>[2x]GSHMDSKHQCVKLNDGHFMPVLGFGTYAPPEVPRSKALEVTKLAIEAGFRHIDSAHLYNNEEQVGLAIRSKIADGSVKREDIFYTSKLWSTFHRPELVRPALENSLKKAQLDYVDLYLIHSPMSLKPGEELSPTDENGKVIFDIVDLCTTWEAMEKCKDAGLAKSIGVSNFNRRQLEMILNKPGLKYKPVCNQVECHPYFNRSKLLDFCKSKDIVLVAYSALGSQRDKRWVDPNSPVLLEDPVLCALAKKHKRTPALIALRYQLQRGVVVLAKSYNEQRIRQNVQVFEFQLTAEDMKAIDGLDRNLHYFNSDSFASHPNYPYSDEY

Human aldo–keto reductase 1C3 (AKR1C3; also known as type 5 17β-hydroxysteroid dehydrogenase, prostaglandin F synthase and 3-α-hydroxysteroid dehydrogenase type 2) is a member of the AKR superfamily of NAD(P)H-dependent oxidoreductases that catalyzes the reduction of a diverse range of carbonyl containing substrates, including exogenous compounds and therapeutic drugs. AKR1C3 functions primarily as a 17-ketosteroid reductase that catalyzes NADPH-dependent reduction of weaker steroid hormones to more potent androgens and estrogens: including the reduction of androstenedione to testosterone, 5α-androstanedione to 5α-dihydrotestosterone (DHT) and estrone to 17β-estradiol. AKR1C3 is overexpressed in prostate cancer and most breast cancer types, which makes it an excellent target for the treatment of hormone-dependent cancers. Gatekeeper residues (W227 and L54) in the steroid channel determine substrate orientation, while the oxyanion site, consisting of the nicotinamide ring from the NAD(P)H cofactor and catalytic residues H117 and Y55, anchors ketone, carboxyl or alcohol containing substrates in proximity to the cofactor for enzymatic reactions.

As can be seen, under the assay conditions used, compound 2 inhibits AKR1C3 reduction of PQ in a sigmoidal, dose-dependent manner, with a resulting calculated IC50 value of ∼7 μM. Compound 2 was found to display selectivity for AKR1C3 over AKR1C2 and was shown to have no off-target affinity for ERα or AR receptors. The structure of AKR1C3·NADP+ in complex with this C-ring fused bile acid tetrazole was determined by X-ray crystallography at 1.4 Å resolution, revealing that the C24 carboxylate is anchored to the catalytic oxyanion site (H117, Y55); meanwhile the tetrazole interacts with a tryptophan (W227) important for steroid recognition. The asymmetric unit comprised two molecules of AKR1C3 with clear electron density for amino acids 6–323 (chain A) and 6–319 (chain B) and the NADP+ cofactor. The electron density corresponding to the 3D structure of compound 2 was clearly visible in the AKR1C3 active site, in both monomer A and monomer B of the asymmetric unit and compound 2 was modeled with full occupancy in both active sites. The overall structure of AKR1C3·NADP+·(2) is globally similar to other AKR1C3 structures, which all contain a characteristic (α/β) 8 – barrel structure, and a highly conserved NADPH cofactor binding site.3,41 However, comparison of known AKR1C3 structures shows that the conformations of amino acid side chains and supporting loop regions involved in ligand binding are dependent on the physico-chemical properties of the bound ligand. Overall, binding of compound 2 to AKR1C3 relies on hydrophobic contacts between its steroidal core and residues lining SP2, including W86, S129, W227 and F311, with support from Y24 in SP3 and F306 in SP1.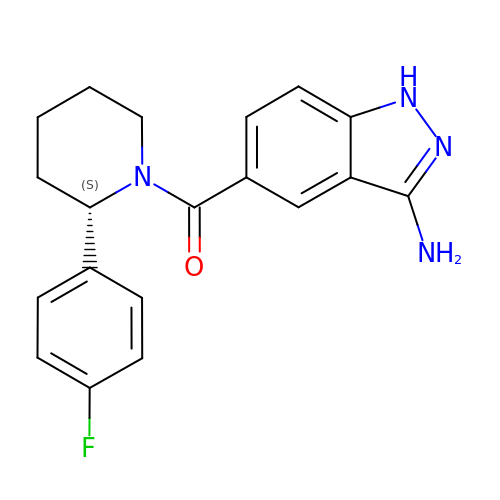(3-amino-1H-indazol-5-yl)[(2S)-2-(4-fluorophenyl)piperidin-1-yl]methanone | C19 H19 F N4 O | VXYMGUGNDZARSZ-KRWDZBQOSA-N>GSHMADSSSSSFFPDFGLLLYLEELNKEELNTFKL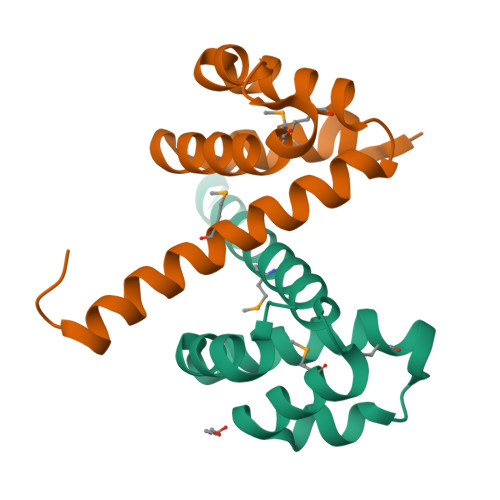FLKETMEPEHGLTPWNEVKKARREDLANLMKKYYPGEKAWSVSLKIFGKMNLKDLCERAKEEINWSAQLE[4x]> MSENERPGLLGRVMSAFKPKAADAVTVASFSQRDAGLYIGSRFTSDAGREVSVQTAMSLDAVQACVKLISQSIAAMPLYLYKKTPDGRKEAVNHPLYDLLLSAPNSSQTAFEFFECILTAMLLHGNAYVRKLMSNGKIESLQFMHSSRLTISQDARGAYKYAYRKLDGTQIDVPSAQVWKIRGYSLDGENGISAIQYGAQVFGTALAAERQAGRAFTNGNLQQIYYSVAAFLTPEQREQFSANVAQSVESGRTPVLEGGIDVKALGLNPADAQ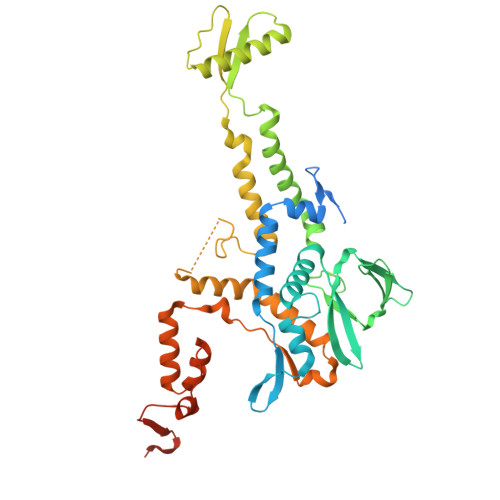LLQSRNYSVESICRFFAVPPSMIGHASAGTTSWGSGIEAQQLAFLGLTLAPWLRRIEQSLSLDLLTPGERRQYFVDYDVTTLLRADSAARSSFYATMVNNGVMTRDECREAEGLPKLGGNASVLTVQSAMVPLDEITNNTGADPAAAQGTTSLDRSAQ N-{(3R)-3-[2-(acetylamino)ethyl]-2-oxo-2,3-dihydro-1H-indol-5-yl}acetamide | C14 H17 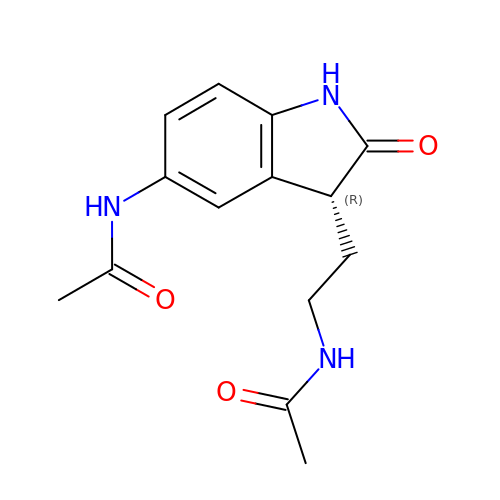N3 O3 | AFKNIIZCTCAFIO-LLVKDONJSA-N>[6x]MKKISLPKIGIRPVIDGRRMGVRESLEEQTMNMAKATAALLTEKLRHACGAAVECVISDTCIAGMAEAAACEEKFSSQNVGLTITVTPCWCYGSETIDMDPTRPKAIWGFNGTERPGAVYLAAALAAHSQKGIPAFSIYGHDVQDADDTSIPADVEEKLLRFARAGLAVASMKGKSYLSLGGVSMGIAGSIVDHNFFESWLGMKVQAVDMTELRRRIDQKIYDEAELEMALAWADKNFRYGEDENNKQYQRNAEQSRAVLRESLLMAMCIRDMMQGNSKLADIGRVEESLGYNAIAAGFQGQRHWTDQYPNGDTAEAILNSSFDWNGVREPFVVATENDSLNGVAMLMGHQLTGTAQVFADVRTYWSPEAIERVTG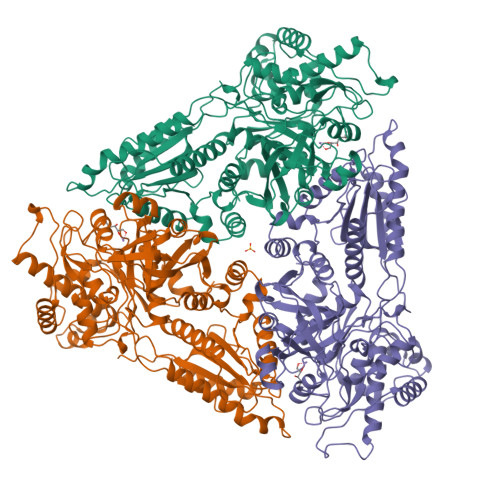HKLDGLAEHGIIHLINSGSAALDGSCKQRDSEGNPTMKPHWEISQQEADACLAATEWCPAIHEYFRGGGYSSRFLTEGGVPFTMTRVNIIKGLGPVLQIAEGWSVELPKDVHDILNKRTNSTWPTTWFAPRLTGKGPFTDVYSVMANWGANHGVLTIGHVGADFITLASMLRIPVCMHNVEETKVYRPSAWAAHGMDIEGQDYRACQNYGPLYKR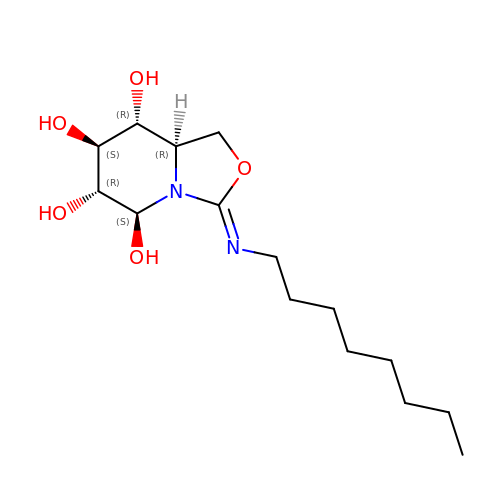(3Z,5S,6R,7S,8R,8aR)-3-(octylimino)hexahydro[1,3]oxazolo[3,4-a]pyridine-5,6,7,8-tetrol | C15 H28 N2 O5 | QJILQIWQVOAQBB-KRIYVDMXSA-N> MVETTQHFVSIESSNRP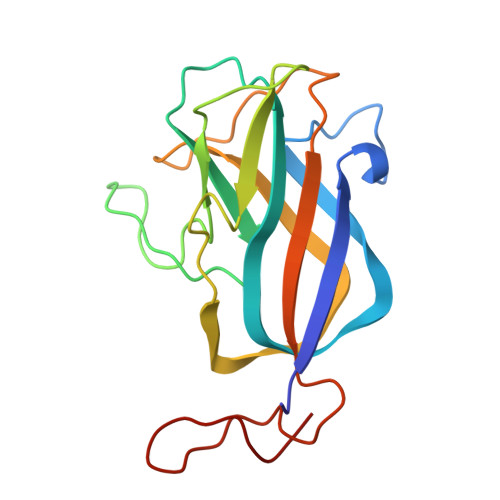DPANTTPANYSIQLPQRYRNIWSAMLVNIALPAVSPPQKYVYLDIDKLNSIDSTSPSGGVNFALAKIPLSIAGTGNVFFADTMTSSFPNVPLQNPVATMDKLNIKLKDANGNVLTIPAGNEHSFMIQLTCGDYIPRGGGSTITQNGRVLGGTR>MAHHHHHHVDDDDKMLVPRGSSGGSTQFYYKLSQELNGDMERVADSLVTLQDQLNSLAAVVLQNRRALDLL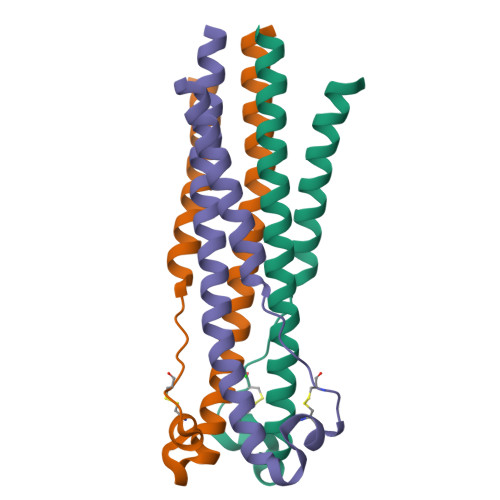TAERGGTCLFLGEECSYYVNQSGIVTEKVKEIRDRIQRRAEELRNT[2x]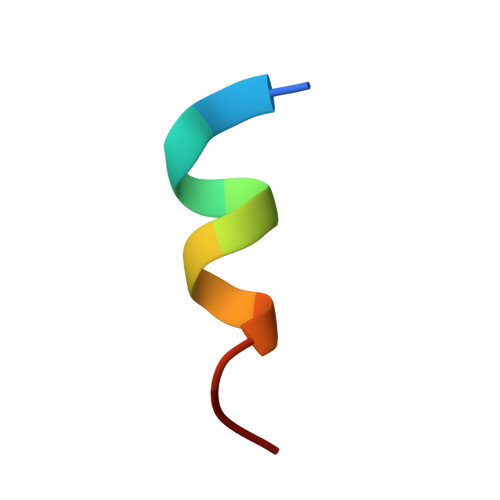> LTFEHYWAQLTS> MDHAPERFDATPPAGEPDRPALGVLELTSIARGITVADAALKRAPSLLLMSRPVSSGKHLLMMRGQVAEVEESMIAAREIAGAGSGALLDELELPYAHEQLWRFLDAPVVADAWEEDTESVIIVETATVCAAIDSADAALK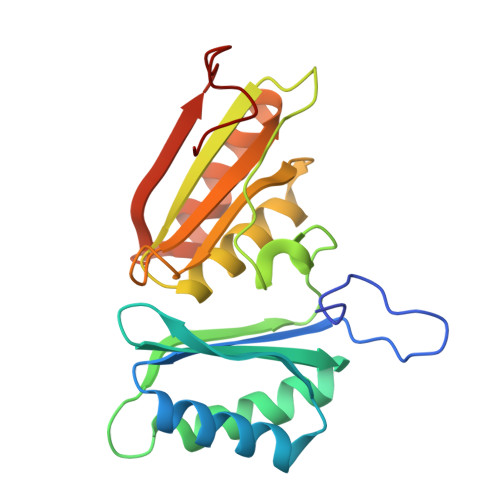TAPVVLRDMRLAIGIAGKAFFTLTGELADVEAAAEVVRERCGARLLELACIARPVDELRGRLFF> GLECDGRTNLCCRQQFFIDFRLIGWNDWIIAPTGYYGNYCEGSCPAYLAGVPGSASSFHTAV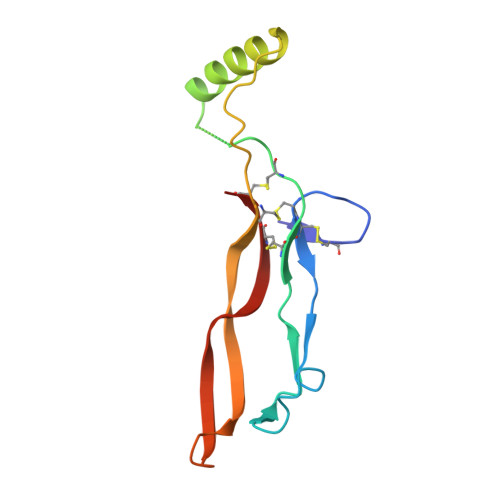VNQYRMRGLNPGTVNSCCIPTKLSTMSMLYFDDEYNIVKRDVPNMIVEECGCA> MAHHHHHHVDDDDKIRDISSKELIKEMNFGWNLGNTMDAQCIEYLNYEKDQTASETCWGNPKTTEDMFKVLIDNQFNVFRIPTTWSGHFGEAPDYKIDEKWLKRVHEVVDYPYKNGAFVILNLHHETWNHAFSETLDTAKEILEKIWSQIAEEFKDYDEHLIFEGLNEPRKNDTPVEWTGGDQEGWDAVNAMNAVFLKTVRSAGGNNPKRHLMIPPYAAACNENSFNNFIFPEDDDKVIASVHAYAPYNFALNNGEGAVDKFDAAGKRDLEWNI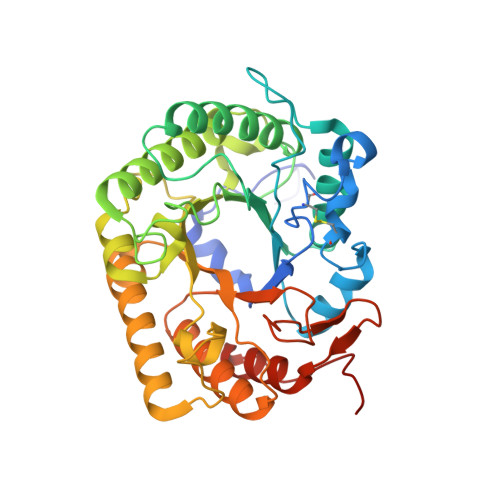NLMKKRFVDQGIPMILGEYGAMNRDNEEDRATWAEFYMEKVTAMGVPQIWWDNGVFEGTGERFGLLDRKNLKIVYPTIVAALQKGRGLEVNVVHAIEKETEE>MKDYSLEIDAVMKAAQINDTNNFVQALMRWHFSKETGSPFWLGMREQLNFDPIKDVKTINDLRQFSDISHCLRQEPVANLVPQGLPADSHPQVYESGGTTGAPKYVVAYDAWIEALISW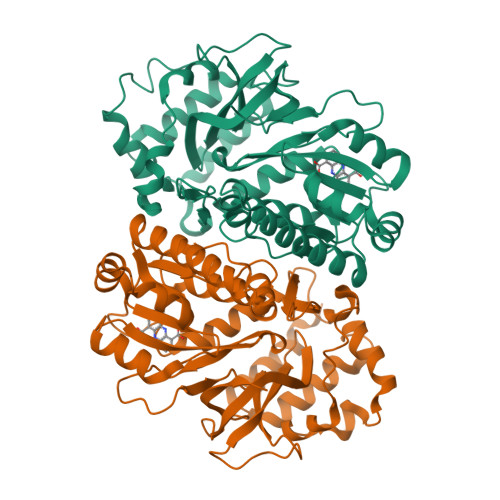RMSGYQHRPGRPSGNTLAAIPTGPHIVGAINKERALRLGGMFFSIDIDPRWVKRSLSEGDTATVRKYTHHLVDQVQNTLMNQDIRFLVTTPPVLRELLKRPEVVLQMKQSLAQITLGGTELNLDEIKFIASEILPDCEFSASYGSTSALGVSRSLLITSESQQVIYDSFSPFITYDVVDSITAQTVEYGERGNVIVTHLSPWAFYPRVAERDTAIRLPGVSGFAGDRLADIEPLKISEGRKVIEGVY[2x]>[2x]MPNNISKSAIIKEGVIIGENVTIEDNVYIDYGCIIRDNVHIK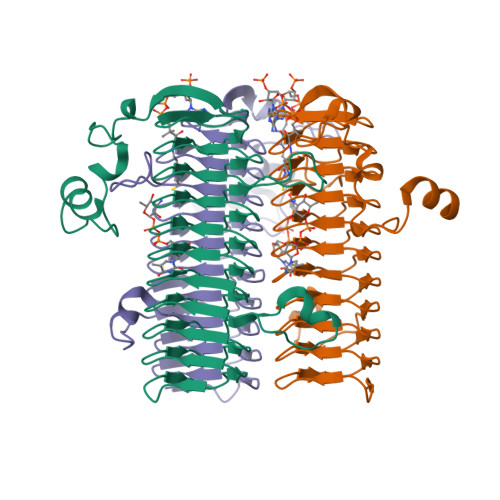KGSFIGARSILGEYLVDFYNDRINKKHPLIIGENALIRTENVIYGDTIIGDNFQTGHKVTIRENTKIGNNVKIGTLSDIQHHVYIGNYVNIHSNVFVGEKSIIKDFVWLFPHVVLTNDPTPPSNELLGVTIELFAVIAARSVVLPGIHINEDALVGAGAVVTKDVPKETVVVGNPAREICSIRKIKNKITGEQVYPWRYTFKRGMPWEETDYDTWIKNISIENLEHHHHHH>[2x]MALFTAKVTARGGRAGHITSDDGVLDFDIVMPNAAAAGQTGTNPEQLFAAGYAACFGG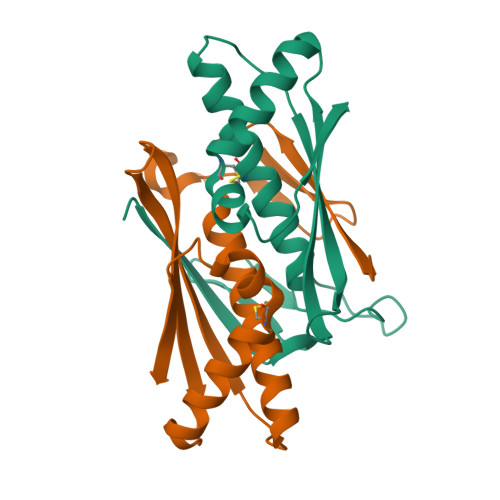ALEHVAKEQNIEIDSEIEGQVSLMKDESDGGFKIGVTLVVNTKDLDREKAQELVNAAHEFCPYSKATRGNVDVKLELK>MNYNAPHRHAVIELSQSAVVHNLKVIKENTHAKEIMAVLKANAFSHGLPEMASLSITAGATRFGMAMLDEALTLRDLGYIQPIDVLGLTDPRYARLAAERNITLAFSTKESIKAAAEQLAGTGLTLKVSLPVDTGLNRIGFKSREDLVAAIQEVSAQDTLIFQSMWTHFATADTPNVDYVDFQ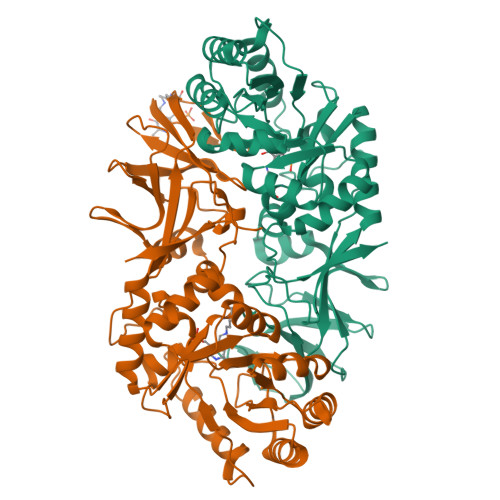ISEWQRLTHDLPVEPNEKHFANTGIATWYPEKINTDIVRLGIGLFGINGSVPIMSMPFELIPALSLKAKVVNSKPLKKGDAVGYGAEYHAPNDGYLITIPIGHSDGYPFNGSGMRALVADGQIGHIVGGVAMDQSMIFVTNPVAVGTTVTLIGRVGDQSITMQDLAEHTQSSIVALMNDFAPRLQRIIVSLEHHHHHH[4x]> DDIKVAVVGAMSGPIAQWGIMEFNGAEQAIKDINAKGGIKGDKLVGVEYDDACDPKQAVAVANKIVNDGIKYVIGHLCSSSTQPASDIYEDEGILMISPGATAPELTQRGYQHIMRTAGLDSSQGPTAAKYILETVKPQRIAIIHDKQQYGEGLARSV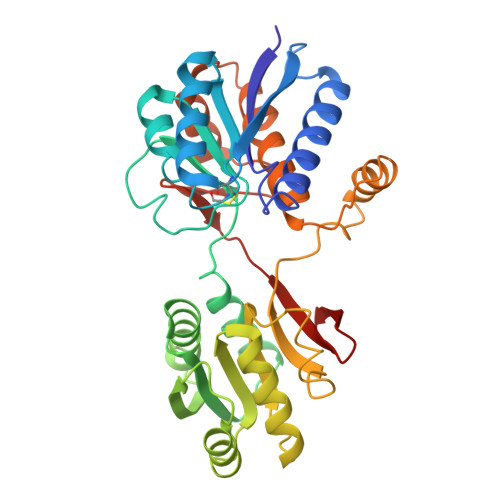QDGLKAANANVVFFDGITAGEKDFSALIARLKKENIDFVYYGGYYPEMGQMLRQARSVGLKTQFMGPEGVGNASLSNIAGDAAEGMLVTMPKRYDQDPANQGIVDALKADKKDPSGPYVWITYAAVQSLATALERTGSDEPLALVKDLKANGANTVIGPLNWDEKGDLKGFDFGVFQWHADGSSTKAK>GPGGSPYLITGIPKDPKHPLPIRKDIDDWYLEQTSAGSNRIQLTLFVEALTVIQNRPLNDQLSYFRLAGIHGAPWTEWDGVPGGQKDSKGNPTGFAVHNNYTFPTWHRVYVTLYEQVIYEAMLDFIKQNVPQNGKADWENEAKQWRLPYWDFARFARHGHDNTQGDELRLPILVTMPMVKVLVPGQPGKQLSKPNPLYRFQMQTLMGTLERPYAITSQKTEEHGWSFDLPFDKCQSTTKYGLLENYNADVWADGGQNWLRANLALNEHPWYQNLDGWDS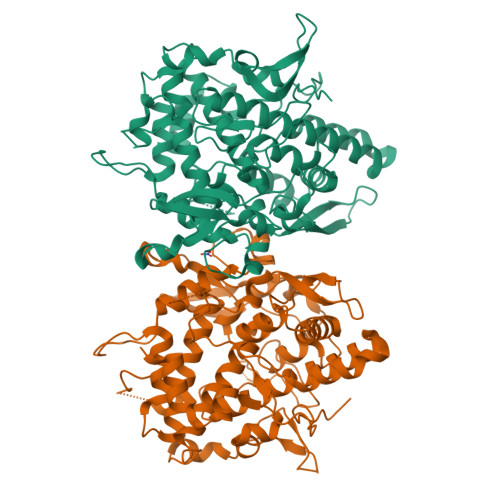VPTLQDMTFRLLTTGGLNWGEFSSTRYDDKKEETQPKNNEQAPKNWMNLEAIHNNVHNWVGGFMFSRPGRHDLKLWGAGHMSSVPVAAYDPIFWLHHCNIDRLTAIWQTVNSGSWFNDDKSKVSKDDDLRPFHRFCEKTRKVVFFRSDDVKDWRSLNYDYAITKDASRIRKEISDLYGQRTK[2x]Septins are present in all mammalian and fungal cellular systems and participate in so diverse intracellular processes such as cytokinesis, polarity establishment or cellular adhesion. They are cytoskeletal guanine nucleotide-binding proteins that belong to the superclass of P-loop NTPases. Instead, septins are scaffolds that recruit other proteins to sites of their activities. Septins assemble into hetero-octameric rods and further into apolar filaments through alternating interactions between two G-domain cores (G-interface) or between two G-domain N- and C-termini (NC-interface), respectively.

Here we present the first X-ray crystal structure of a tetrameric Shs1-Cdc12-Cdc3-Cdc10 complex at a resolution of 3.2 Å. We removed the unstructured extensions from all four subunits and coexpressed Shs1G21-S339-Cdc12M1-G314-Cdc3Q81-A410-Cdc10G30-R322 together in E. coli. G-interfaces are formed between Shs1 and Cdc12 as well as between Cdc3 and Cdc10. Cdc12 and Cdc3 are connected by a NC-interface. All subunits contain GDP without a coordinated Mg2+ ion. However, a filament-like structure with the subunit arrangement Shs1-Cdc12-Cdc3-Cdc10:Shs1-Cdc12-Cdc3-Cdc10 can be generated, indicating that the crystallization conditions favored the formation of a non-native Cdc10-Shs1 interface. Cdc10 lacks the α0-helix in our expression construct, explaining the tetrameric nature of the complex. The switch 1 loop of Shs1 is longer than in the other canonical septins and is – except Shs1H51 and Shs1K52 - not in contact with the nucleotide. Instead, it snuggles along the surface of the Shs1 subunit where it folds into an interrupted β-strand between V68 and N80 which is attached to the β2-strand of the central β-sheet. All septins possess a highly conserved arginine in the SUE β-meander (Arg(βb)), representing the central element of an overall conserved interaction hub in the nucleotide-binding pocket.

> MADLNWMGFQFNIMVVGQSGLGKSTLINTLFASHLIDSATGDDISALPVTKTTEMKISTHTLVEDRVRLNINVIDTPGFGDFIDNSKAWEPIVKYIKEQHSQYLRKELTAQRERFITDTRVHAILYFLQPNGKELSRLDVEALKRLTEIANVIPVIGKSDTLTLDERTEFRELIQNEFEKYNFKIYPYDSEELTDEELELNRSVRSIIPFAVVGSENEIEINGETFRGRKTRWSAINVEDINQCDFVYLREFLIRTHLQDLIETTSYIHYEGFRARQLIALKENANSRSSAHMSSNAIQR;> MLQVLPDQPEIKFIRRQINGYVGFANLPKQWHRRSIKNGFSFNLLCVGPDGIGKTTLMKTLFNNDDIEANLVKDYEEELANDQEEEEGQGEGHENQSQEQRHKVKIKSYESVIEENGVKLNLNVIDTEGFGDFLNNDQKSWDPIIKEIDSRFDQYLDAENKINRHSINDKRIHACLYFIEPTGHYLKPLDLKFMQSVYEKCNLIPVIAKSDILTDEEILSFKKTIMNQLIQSNIELFKPPIYSNDDAENSHLSERLFSSLPYAVIGSNDIVENYSGNQVRGRSYPWGVIEVDNDNHSDFNLLKNLLIKQFMEELKERTSKILYENYRSSKLA;> MGSSHHHHHHSQDPNSMSAATATAAPVPPPVGISNLPNQRYKIVNEEGGTFTVMLCGESGLGKTTFINTLFQTVLKRADGQQHRQEPIRKTVEIDITRALLEEKHFELRVNVIDTPGFGDNVNNNKAWQPLVDFIDDQHDSYMRQEQQPYRTKKFDLRVHAVLYFIRPTGHGLKPIDIETMKRLSTRANLIPVIAKADTLTAQELQQFKSRIRQVIEAQEIRIFTPPLDADSKEDAKSGSNPDSAAVEHARQLIEAMPFAIVGSEKKFDNGQGTQVVARKYPWGLVEIENDSHCDFRKLRALLLRTYLLDLISTTQEMHYETYRRLRLEG;> MGITYTMLLCGPAGTGKTAFANNLLETKIFPHKYQYGKSNASISSNPEVKVIAPTKVVSFNSKNGIPSYVSEFDPMRANLEPGITITSTSLELGGNKDQGKPEMNEDDTVFFNLIMTHGIGENLDDSLCSEEVMSYLEQQFDIVLAEETRIKRNPRFEDTRVHVALYFIEPTGHGLREVDVELMKSISKYTNVLPIITRADSFTKEELTQFRKNIMFDVERYNVPIYKFEVDPEDDDLESMEENQALASLQPFAIITSDTRDSEGRYVREYPWGIISIDDDKISDLKVLKNVLFGSHLQEFKDTTQNLLYENYRSEKLSS>[3x]QLTTESMPFNVAEGKEVLLLVHNLPQQLFGYSWYKGERVDGNRQIVGYAIGTQ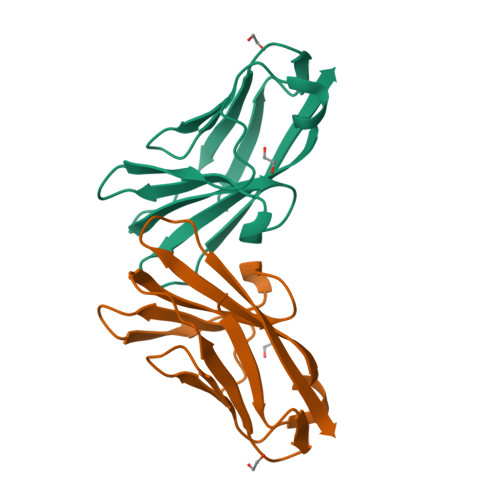QATPGPANSGRETIYPNASLLIQNVTQNDTGFYTLQVIKSDLVNEEATGQFHVY> MDILKEKIDVASRLYNLNLDHIPATLQVIEHAMLLLKNNAGYGYFGSFNGKNTQEYHSFTFNGEYSRPVRDDLFITDYDFFVSGFREFNESLRDIGSKWSSFDSRRANKIIYTSVMSVACCFDLWKSGSRKTPGTFFEIFMAAVLKWMIP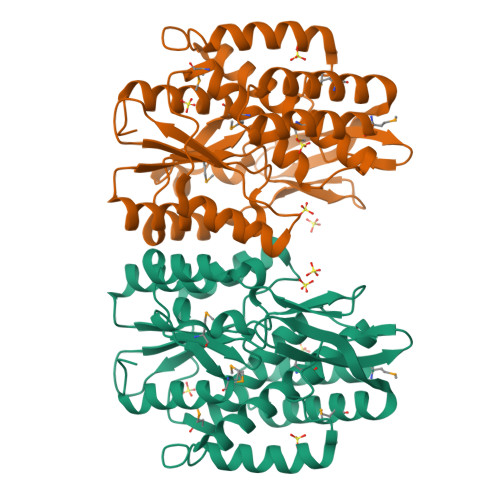DEIFSKHIPLIDQLESDDESIDPSSVSTDIVIKSAYANASVVIPLKITTRERIVQPFAQQRILDSYFGNGVYFSFLACISETQQDKKKKKVNHICVPGTIRLYQKYLSSLSGMYYCDIPERYLERDLTDIIPVRTMGDFLFDIYSFFRSQGAAALEHHHHHH> SMGGKKFQAMPQLPSTVLDRVFEQARQQPEAIALRRCDGTSALRYRELVAEVGGLAADLRAQSVSRGSRVLVISDNGPETYLSVLACAKLGAIAVMADGNLPIAAIE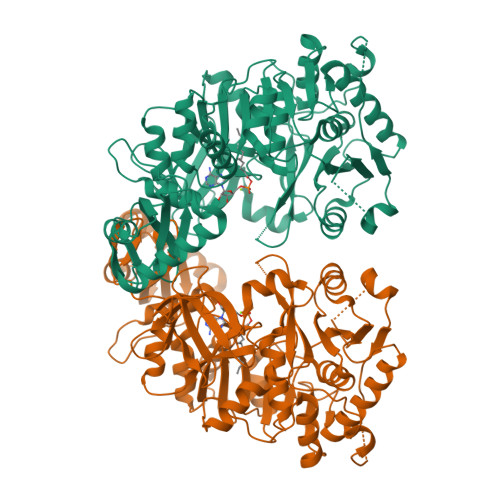RFCQITDPAAALVAPGSKMASSAVPEALHSIPVIAVDIAAVTRESEHSLDAASLAGNADQGSEDPLAMIFTSGTTGEPKAVLLANRTFFAVPDILQKEGLNWVTWVVGETTYSPLPATHIGGLWWILTCLMHGGLCVTGGENTTSLLEILTTNAVATTCLVPTLLSKLVSELKSANATVPSLRLVGYGGSRAIAADVRFIEATGVRTAQVYGLSETGCTALCLPTDDGSIVKIEAGAVGRPYPGVDVYLAATDGIGPTAPGAGPSASFGTLWIKSPANMLGYWNNPERTAEVLIDGWVNTGDLLERREDGFFYIKGRSSEMIICGGVNIAPDEVDRIAEGVSGVREAACYEIPDEEFGALVGLAVVASAELDESAARALKHTIAARFRRESEPMARPSTIVIVTDIPRTQSGKVMRASLAAAATADKARVVVRG> MYKSVNITFELDERIDKVLNEKCSAYTVELGTEVNEFACVVADAVIKTLQPVSELLTPLGIDLDEWSMA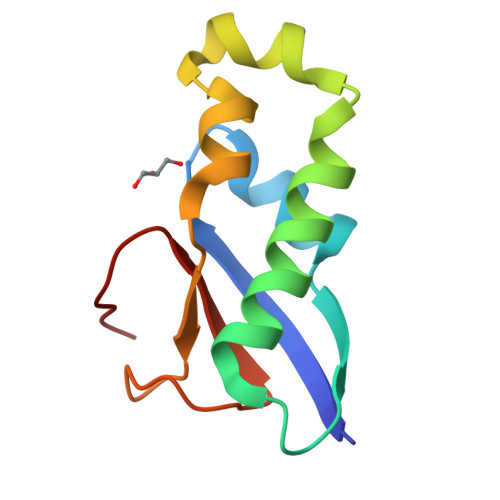TYYLFDESGEFKLASHMYCSFYLEHHH> SMTEEERSSALSEVSLRLLCHDDIDTVKHLCGDWFPIEYPDSWYRDITSNKKFFSLAATYRGAIVGMIVAEIKNRTKIHKEDGDILASNFSVDTQVAYILSLGVVKEFRKHGIGSLLLESLKDHISTTAQDHCKAIYLHVLTTNNTAINFYENRDFKQHHYLPYYYSIRGVLKDGFTYVLYINGGHPPWTILDYIQHLGS

As the first N-terminal acetyltransferase discovered on an organelle, NatF, encoded by NAA60 and also named as Histone acetyltransferase type B protein 4 (HAT4), Naa60 or N-acetyltransferase 15 (NAT15), is the youngest member of the NAT family. As an N-terminal acetyltransferase, NatF can specifically catalyze acetylation of the N-terminal α-amine of most transmembrane proteins and has substrate preference towards proteins with Met-Lys-, Met-Val-, Met-Ala- and Met-Met-N-termini, thus partially overlapping substrate selectivity with NatC and NatE18. Another important feature of NatF is that this protein is anchored on the Golgi apparatus through its C-terminal membrane-integrating region and takes part in the maintaining of Golgi integrity. The structure of hNaa60 protein contains a central domain exhibiting a classic GCN5-related N-acetyltransferase (GNAT) folding, along with the extended N- and C-terminal regions.

The crystal structures of hNaa60(1-242)/Ac-CoA and hNaa60(1-199)/CoA were determined by molecular replacement and refined to 1.38 Å and 1.60 Å resolution, respectively. In the hNaa60(1-199)/CoA structure, a part of the α5-helix is deleted due to truncation of the C-terminal region. Interestingly, the remaining residues in α5-helix still form an amphipathic helix although the hydrophobic interaction with the N-terminal hydrophobic groove of a neighbor molecule is abolished and the helix is largely exposed in solvent due to different crystal packing. Upon removing the C-terminal region of hNaa60, we observed that hNaa60 (1-199) molecules pack in a different way involving the β7-β8 hairpin in the crystal, leading to about 50 degree rotation of the hairpin which moves away from the α1-α2 loop. Interestingly, in the hNaa60(1-199) crystal structure, the displaced β7-β8 hairpin opened a second way for the substrate to access the active center that would readily accommodate the binding of the H4 peptide, thus implied a potential explanation for KAT activity of this enzyme from a structural biological view. However, since hNaa60(1-242) and hNaa60(1-199) were crystallized in different crystal forms, the observed conformational change of the β7-β8 hairpin may simply be an artifact related to the different crystal packing. The electron density of Phe 34 side-chain is well defined in the hNaa60(1-242)/Ac-CoA structure, but becomes invisible in the hNaa60(1-199)/CoA structure, indicating displacement of the Phe 34 side-chain in the latter. Interestingly, in the structure of hNaa60(1-199)/CoA, the terminal thiol of CoA adopts alternative conformations. One is to approach the substrate amine (as indicated by the superimposed hNaa50/CoA/peptide structure), similar to the terminal ethanethioate of Ac-CoA in the structure of hNaa60(1-242)/Ac-CoA; the other is to approach the α1-α2 loop and away from the substrate amine.>[2x]MFQPLLDAYVESASIEKMASKSPPPLKIAVANWWGDEEIKEFKNFVLYFILSQRYTITLHQNPNEFSDLVFGNPLGSARKILSYQNAKRVFYTGENESPNFNLFDYAIGFDELDFNDRYLRMPLYYNELHIKAESVNDTTAPYKLKDNSLYALKKPSHCFKEKHPNLCAVVNDESDPLKRGFASFVASNPNAPIRNAFNDALNSIEPVTGGGSVRNTLGYNVKNKNEFLSQY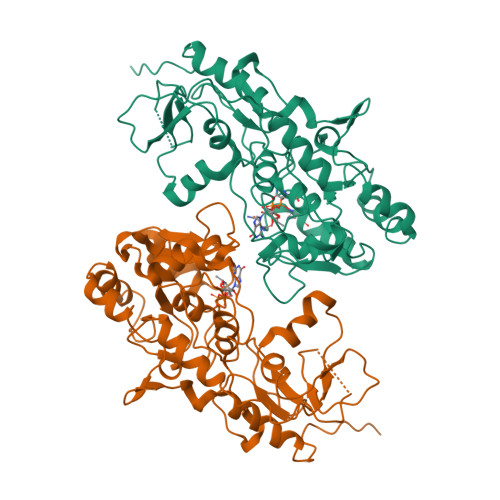KFNLCFENTQGYGYVTEKIIDAYFSHTIPIYWGSPSVAKDFNPKSFVNVHDFKNFDEAIDYIKYLHTHKNAYLDMLYENPLNTLDGKAYFYQNLSFKKILAFFKTILDNDTIYHDNPFIFCRDLNEPLVTIDDLRANYDDLRVNYDDLRINYDDLRVNYDDLRINYDDLRVNYDDLRVNYLEHHHHHH>GSPRTVEEIFKDYSARRAALLRALTKDVDDFY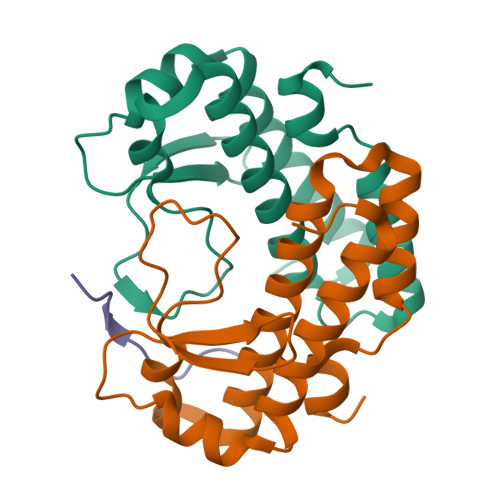SQCDPEKENLCLYGHPNESWEVNLPAEEVPPELPEPALGINFARDGMQRKDWLSLVAVHSDCWLLSVSFYFGARLNRNERKRLFSLINDLPTLFDVVTGRKAM[4x];>ILAWGRGGTRSNTR[2x]> GPMPKPINVRVTTMDAELEFAIQPNTTGKQLFDQVV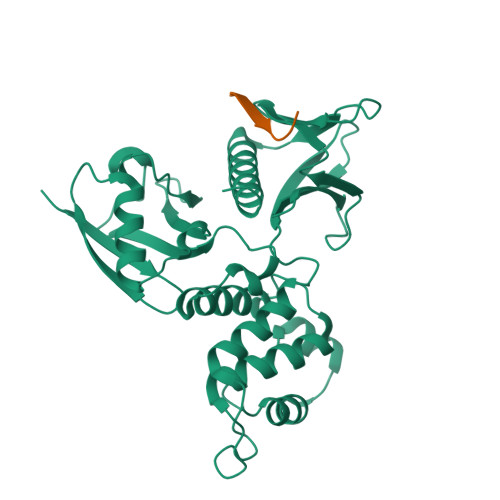KTVGLREVWFFGLQYVDSKGYSTWLKLNKKVTQQDVKKENPLQFKFRAKFFPEDVSEELIQEITQRLFFLQVKEAILNDEIYCPPETAVLLASYAVQAKYGDYNKEIHKPGYLANDRLLPQRVLEQHKLTKEQWEERIQNWHEEHRGMLREDSMMEYLKIAQDLEMYGVNYFEIKNKKGTELWLGVDALGLNIYEHDDKLTPKIGFPWSEIRNISFNDKKFVIKPIDKKAPDFVFYAPRLRINKRILALCMGNHELYMRRRKPDTIEVQQMKAQAR;> SRRRCGQKKKLVINGGNGTV>LLPILSFPDPRLRTIAKPVEEVTDEIRQLAADMFETMYAAPGIGLAASQVDRHIQLIVMDLSESKDEPMVFINPKVTPLTEETQPYEEGCLSVPQIYDKVDRPSRVKIEAINLEGQAFEIEADGLLAVCIQHEM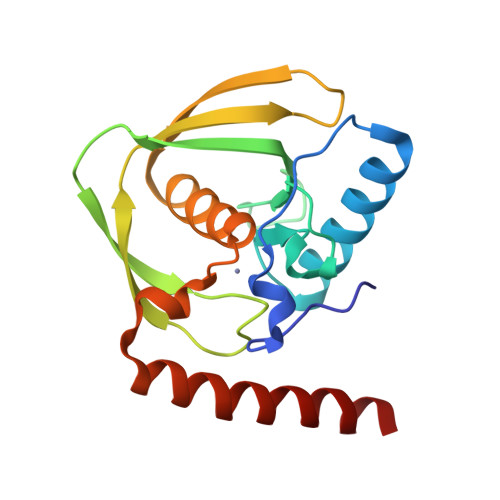DHLNGKLFVDYLSPLKRQRAREKVEKIVRQREREKV[2x]>[6x]MLDNLLRHLKISKEQITPVVLVVGDPGRVDKIKVVCDSYVDLAYNREYKSVECHYKGQKFLCVSHGVGSAGCAVCFEELCQNGAKVIIRAGSCGSLQPDLIKRGDICIC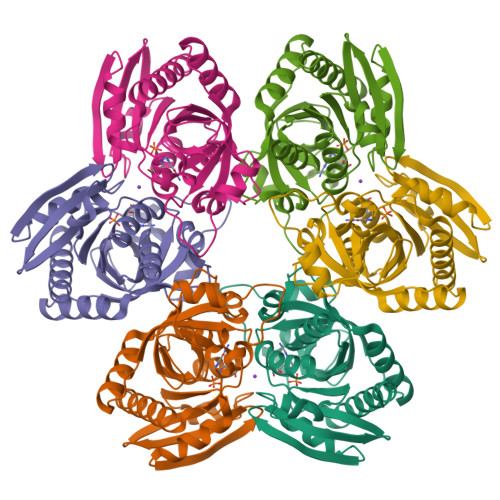NAAVREDRVSHLLIHGDFPAVGDFDVYDTLNKCAQELNVPVFNGISVSSDMYYPNKIIPSRLEDYSKANAAVVEMELATLMVIGTLRKVKTGGILIVDGCPFKWDEGDFDNNLVPHQLENMIKIALGACAKLATKYAKGEFEAYVEQKLISEEDLNSAVDHHHHHH>[2x]MDDLTIEILTDDADYDLQRFDCGEEALNLFLTTHLVRQHRNKILRAYILCRNTPERQVLGYYTLCGSCFERAALPSKSKQKKIPYKNIPSVTLGRLAIDRSLQGQGWG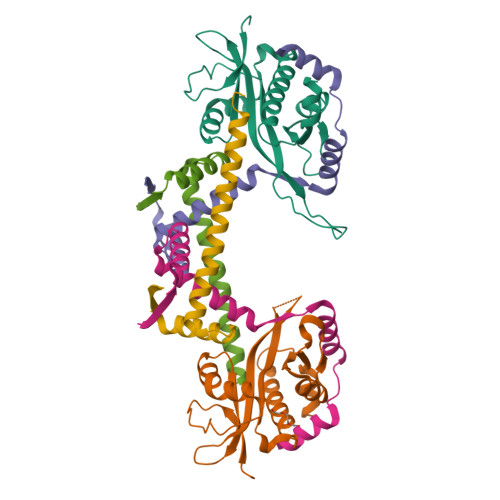ATLVAHAMNVVWSASLAVGIHGLFVEALNEKAHTFYKSLGFIPLVGENENALFFPTKSIELLFTQSDLEHHHHHH;>[4x]MSAVKKQRIDLRLTDDDKSMIEEAAAISNQSVSQFMLNSASQRAAEVIEQHRRVILNEESWTRVMDALSNPPSPGEKLKRAAKRLQGM>[2x]GSHMQQWVDCEFTGRDFRDEDLSRLHTERAMFSECDFSGVNLAESQHRGSAFRNCTFERTTLWHS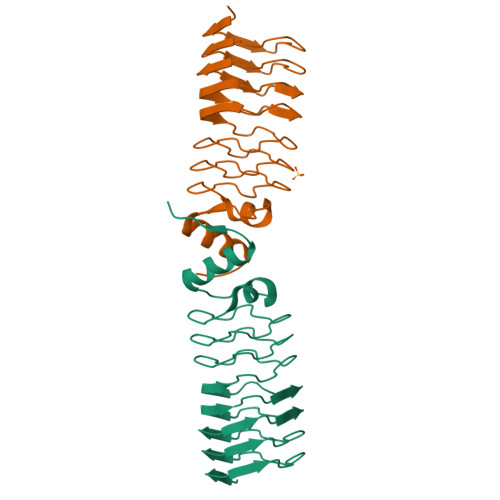TFAQCSMLGSVFVACRLRPLTLDDVDFTLAVLGGNDLRGLNLTGCRLRETSLVDTDLRKCVLRGADLSGARTTGARLDDADLRGATVDPVLWRTASLVGARVDVDQAVAFAAAHGLCLAGG> MMFGKKKNNGGSSTARYSAGNKYNTLSNNYALSAQQLLNASKIDDIDSMMGFERYVPPQYNGRFDAKDIDQIPGRVGWLTNMHATLVSQETLSSGSNGGGNSNDGERVTTNQGISGVDFYFLDEEGGSFKSTVVYDPYFFIACNDESRVNDVEELVKKYLESCLKSLQIIRKEDLTMDNHLLGLQKTLIKLSFVNSNQLFEARKLLRPILQDNANNNVQRNIYNVAANGSEKVDAKHLIEDIREYDVPYHVRVSIDKDIRVGKWYKVTQQGFIEDTRKIAFADPVVMAFDIETTKPPLKFPDSAVDQIMMISYMIDGEGFLITNREIISEDIEDFEYTPKPEYPGFFTIFNENDEVALLQRFFEHIRDVRPTVISTFNGDFFDWPFIHNRSKIHGLDMFDEIGFAPDAEGEYKSSYCSHMDCFRWVKRDSYLPQGSQGVKAVTQSKLGYNPIELDPELMTPYAFEKPQHLSEYSVSDAVATYYLYMKYVHPFIFSLCTIIPLNPDETLRKGTGTLCEMLLMVQAYQHNILLPNKHTDPIERFYDGHLLESETYVGGHVESLEAGVFRSDLKNEFKIDPSAIDELLQELPEALKFSVEVENKSSVDKVTNFEEIKNQITQKLLELKENNIRNELPLIYHVDVASMYPNIMTTNRLQPDSIKAERDCASCDFNRPGKTCARKLKWAWRGEFFPSKMDEYNMIKRALQNETFPNKNKFSKKKVLTFDELSYADQVIHIKKRLTEYSRKVYHRVKVSEIVEREAIVCQRENPFYVDTVKSFRDRRYEFKGLAKTWKGNLSKIDPSDKHARDEAKKMIVLYDSLQLAHKVILNSFYGYVMRKGSRWYSMEMAGITCLTGATIIQMARALVERVGRPLELDTDGIWCILPKSFPETYFFTLENGKKLYLSYPCSMLNYRVH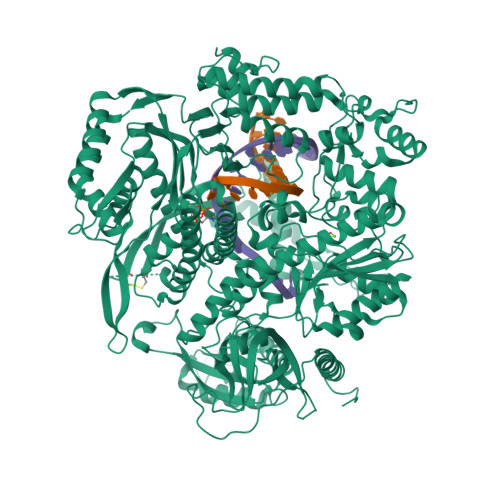QKFTNHQYQELKDPLNYIYETHSENTIFFEVDGPYKAMILPSSKEEGKGIKKRYAVFNEDGSLAELKGFELKRRGELQLIKNFQSDIFKVFLEGDTLEGCYSAVASVCNRWLDVLDSHGLMLEDEDLVSLICENRSMSKTLKEYEGQKSTSITTARRLGDFLGEDMVKDKGLQCKYIISSKPFNAPVTERAIPVAIFSADIPIKRSFLRRWTLDPSLEDLDIRTIIDWGYYRERLGSAIQKIITIPAALQGVSNPVPRVEHPDWLKRKIA> MNRLLNEKVEEFKKGVLKAGWFIEKMFRNSISSLVERNESLAREVIADEEVVDQMEVEIQEKAMEVLGLFSPIGKPLLTVTAGIRVAELIENIADKCHDIAKNVLELMEEPPLKPLEDIPAMANQTSEMLKFALRMFADVNVEKSFEVCR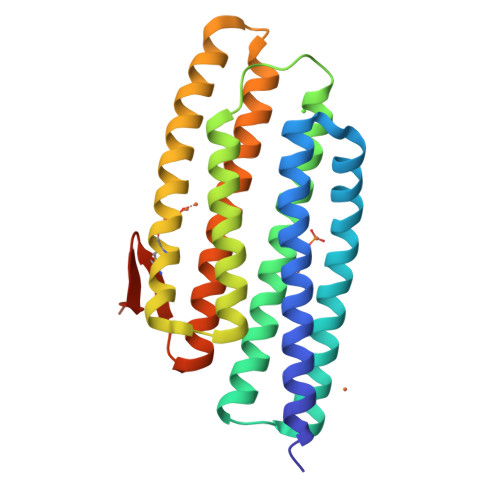MDSKVDDLYEKVREELLLYMMESPKYVKRALLLLEIAGNIEIIADYATNIVEVSVYMVQGEAYKCYHDELLLFKKSGGVLFESSD5-[4-(2-DIMETHYLAMINOETHYLOXY)PHENYL]-2-UREIDO-THIOPHENE-3-CARBOXAMIDE | C16 H20 N4 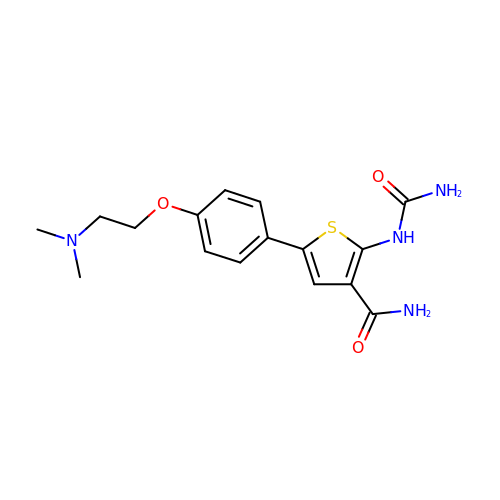O3 S | RFSVVCBVIFWEMZ-UHFFFAOYSA-N>GSHMVRNVDVKSRIMDQYADWKGVRYRLGGSTKKGIDSSGFVQRTFRE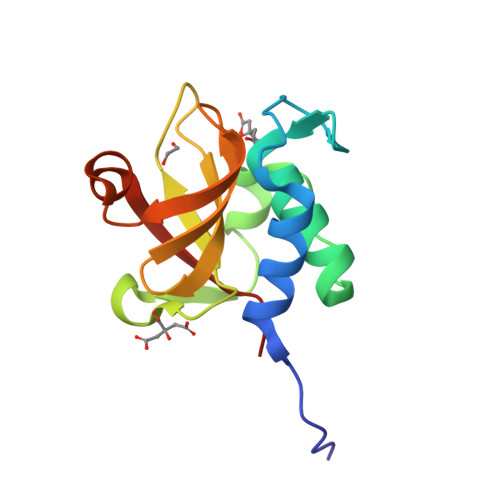QFGLELPRSTYEQQEMGKSVSRSNLRTGDLVLFRAGSTGRHVGIYIGNNQFVHASTSSGVIISSMNEPYWKKRYNEARRVLSRS[2x]2-naphthalen-2-yl-~{N}-pyridin-2-yl-ethanamide 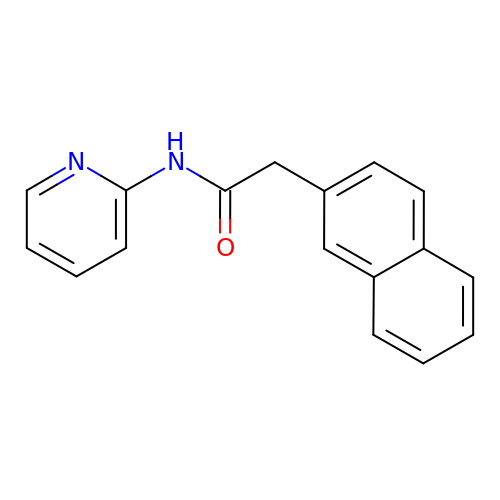| C17 H14 N2 O | KXZCFXKLOSDNKK-UHFFFAOYSA-N2-BUTANOL | C4 H10 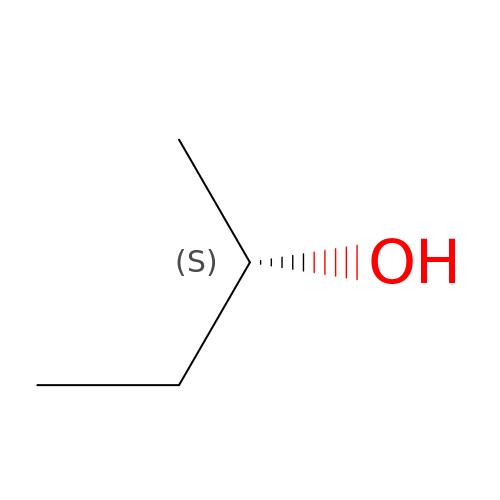O | BTANRVKWQNVYAZ-BYPYZUCNSA-N> GAMGSAVSESQLKKMVSKYKYRDLTVRETVNVITLYKDLKPVLDSYGTGSRELMNLTGTIPVPYRGNTYNIPICLWLLDTYPYNPPICFVKPTSSMTIKTGKHVDANGKIYLPYLHEWKHPQSDLLGLIQVMIVVFGDEPPVFSRP;> PTPSA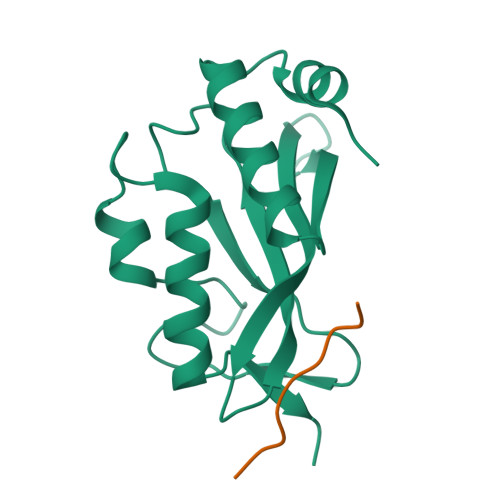PVPL>[6x]MSMADRDGVIWYDGELVQWRDATTHVLTHTHHYGMGVFEGVRAYDTPQGTAIFRLQAHTDRLFDSAHIMNMQIPYSRDEINEATRAAVRENNLESAYIRPMVFYGSEGMGLRASGLKVHVIIAAWSWGAYMGEEALQQGIKVRTSSFTRHHVNISMTRAKSNGAYINSMLALQEAISGGADEAMMLDPEGYVAEGSGENIFIIKDGVIYTPEVTACLNGITRNTILTLAAEHGFKLV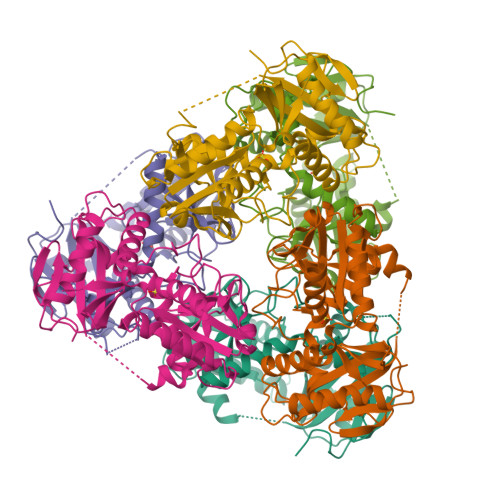EKRITRDEVYIADEAFFTGTAAEVTPIREVDGRKIGAGRRGPVTEKLQKAYFDLVSGKTEAHAEWRTLVK>YFGKLESKLSVIRNLNDQVLFIDQGNRPLFEDMTDSDCRDNAPRTIFIISMYKDSQPRGMAVTISVKCEKISTLSCENKIISFKEMNPPDNIKDTKSDIIFFQRSVPGHDNKMQFESSSYEGYFLACEKERDLFKLILKKEDELGDRSIMFTVQNED[4x]

Interleukin (IL)-18 belongs to the IL-1 superfamily and was first discovered as an interferon gamma (IFN-γ)-inducing factor in sera from mice with hepatitis stimulated with Propionibacterium acnes and lipopolysaccharide1. This proinflammatory cytokine is secreted by various types of cells and strongly augments IFN-γ production in type-1 helper T (Th1) cells and natural killer (NK) cells following activation of NK-cell cytotoxicity; thus, it plays a critical role in inflammation and the host defense against microbes. IL-18/IL-18Rα/IL-18Rβ ternary complex formation juxtaposes the intracellular Toll-Interleukin-1 receptor domains of IL-18Rα and IL-18Rβ, to which the adaptor molecule myeloid differentiation factor 88 (MyD88) is recruited presumably with the aid of TRAM6. We determined the crystal structures of IL-18, the IL-18/IL-18Rα binary complex and the IL-18/IL-18Rα/IL-18Rβ signalling ternary complex at the resolutions 2.33, 3.10 and 3.10 Å, respectively.

The IL-18 structure essentially does not change on complex formation, maintaining the β-trefoil fold that comprises 12 β-strands (β1-β12) and 2 α-helices (α1-α2), as previously reported19. Our previous NMR study showed that the residues 34 to 42 are flexible despite partial α-helix formation in this region (residues 38–41). In addition, two isomeric forms that originate from a cis or trans peptide bond between Ala42IL-18-Pro43IL-18 in the loop are equally populated in the solution structure. The flexible nature of the segment produces a variety of architectures, as demonstrated in several crystallographic reports, including a loop with a trans isomer22, an α-helix with a cis isomer21 or, primarily, unobservable flexible loop with a trans isomer2022.(4~{R})-6-[(~{E})-5-(7-methoxy-3,4-dihydro-2~{H}-quinolin-1-yl)pent-1-enyl]-4-methyl-8-morpholin-4-ylcarbonyl-1,3,4,5-tetrahydro-1,5-benzodiazepin-2-one | C30 H38 N4 O4 | 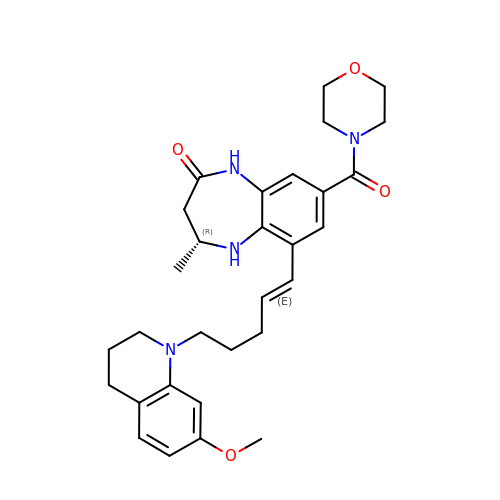YARRLUKCMVZYJK-HXRGIAOBSA-N> MIDKSAFVHPTAIVEEGASIGANAHIGPFCIVGPHVEIGEGTVLKSHVVVNGHTKIGRDNEIYQFASIGEVNQDLKYAGEPTRVEIGDRNRIRESVTIHRGTVQGGGLTKVGSDNLLMINAHIAHDCTVGNRCILANNATLAGHVSVDDFAIIGGMTAVHQFCIIGAHVMVGGCSGVAQDVPPYVIAQGNH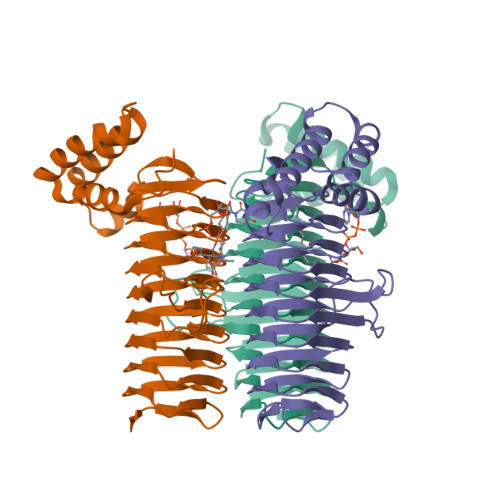ATPFGVNIEGLKRRGFSREAITAIRNAYKLIYRSGKTLDEVKPEIAELAETYPEVKAFTDFFARSTRGLIR We report structures of the Mycobacterium tuberculosis isoprenyl diphosphate synthase Rv2173 in three forms: apo and two substrate-bound forms [isoprenyl diphosphate (IPP) and dimethylallyl diphosphate (DMAPP)]. The protein possesses a canonical all-α-helical trans-isoprenyl diphosphate synthase fold that is dimeric in each form. Two divalent-metal-binding aspartic acid-rich DDxxD motifs termed the FARM and SARM (first and second aspartic acid-rich DDxxD motifs) are important in all-E-prenyltransferase mechanisms. Rv2173 is a homodimer with a canonical class I diterpene synthase fold, with structural analysis identifying some conserved mechanistic features in C-terminal closure and supporting its annotation as a short-chain (C10–C15) product-length synthase.

The IPP-bound structure appears to be the most closed form with a fully ordered C-terminus. It has three metal ions bound: two to the FARM unit (DDLID; residues 84–88) and one near the SARM unit (DDVLGVFGD; residues 236–244), with the IPP occupying the putative allylic/DMAPP site, coordinating all three metal ions and making interactions with Lys194 and Lys260. While surprising, there is precedent for IPP binding to the allylic/DMAPP site in other E-prenyltransferases. Variations in the FARM and SARM motifs have been proposed to influence how the metals coordinate; however, it is important to note that IPP is not the physiological ligand for the metal-associated allylic binding site. We observe a role for Phe232 from this site in changes associated with C-terminal closure in the IPP-bound structure. In this structure, Arg350 faces into the active site and forms hydrogen-bonding interactions with the final C-terminal residue Ala352, as well as Asp236 from the SARM motif and the backbone of Phe232. Although limited conservation suggests that this mechanism is unlikely to be fully preserved in Rv2173, these three residues (Arg350/FPPSArg351; Phe232/FPPSPhe239; Asp236/FPPSAsp243) are conserved, correlating with their potential shared importance. The apo structure was solved with a dimer in the asymmetric unit in space group P21212, while both substrate-bound structures were solved in space group I222 with monomers in the asymmetric unit, generating dimers on the application of crystallographic symmetry.

> MSYYHHHHHHLESTSLYKKAGSAAALFRFKKEPFTMAGAITDQLRRYLHGRRRAAAHMGSDYDGLIADLEDFVLGGGKRLRPLFAYWGWHAVASREPDPDVLLLFSALELLHAWALVHDDLIDRSATRRGRPTAQLRYAALHRDRDWRGSPDQFGMSAAILLGDLAQVWADDIVSKVCQSALAPDAQRRVHRVWADIRNEVLGGQYLDIVAEASAAESIESAMNVATLKTACYTVSRPLQLGTAAAADRSDVAAIFEHFGADLGVAFQLRDDVLGVFGDPAVTGKPSGDDLKSGKRTVLVAEAVELADRSDPLAAKLLRTSIGTRLTDAQVRELRTVIEAVGARAAAESRIAALTQRALATLASAPINATAKAGLSELAMMAANRSA>[2x]MTKKGDTYNEAWVKDTNGFDILMGQFAHNIENIWGFKEVVIAGPKDYVKYTDQYQTRSHINFDDGTITIETIAGTEPAAHLRRAIIKTLLMGDDPSSVDLYSDVDDITISKEPFLYGQVVDNTGQPIRWEGRASNFADYLLKNRLKSRSNGLRIIYSVTINMVPNHLDKRAHKYLGMVRQASRKYGVDESLILAIMQTESSFNPYAVSRSDALGLMQVVQHTAGKDVFRSQGKSGTPSRSF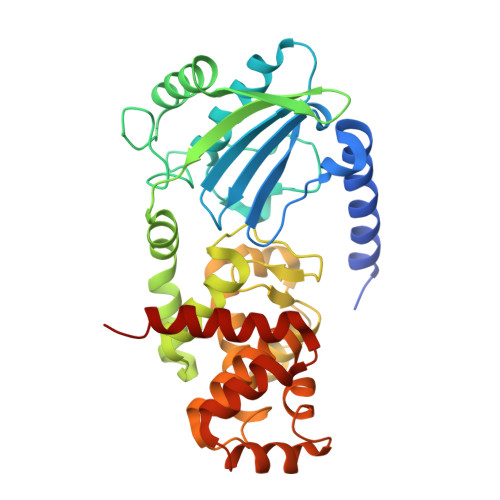LFDPASNIDTGTAYLAMLNNVYLGGIDNPTSRRYAVITAYNGGAGSVLRVFSNDKIQAANIINTMTPGDVYQTLTTRHPSAESRRYLYKVNTAQKSYRRR> GPDSMASSSTAYYLKDAGFHIRNIPKAWNDWNLFHVFQNFGKVSYCRV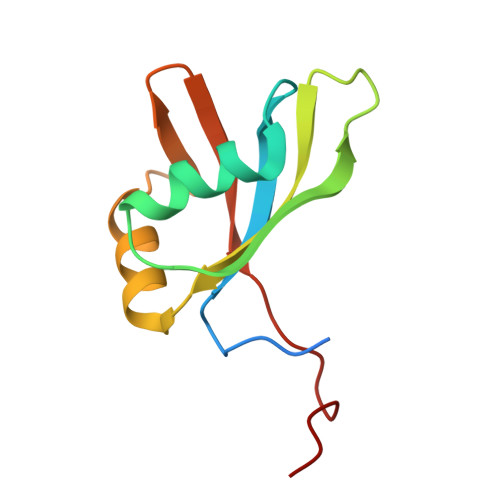VGQSNDGQVQLGFVNMMSVADADEVRKNLNDGNLIGENFTLKVTDHKNVGGSLLP>GSHMIARIIGEIGIEGARFIEENIDEQFKALRYLSKGIDSETFVKLVIANSLVSYQLTGKGEQWWWEFAKYFYGRDVKSIYLAYKEFLPNSRFNRRLIPQKLSRIRRVETFLSTLTEERIEEYYGDMSSLWGSIARALGVDKESKTVVF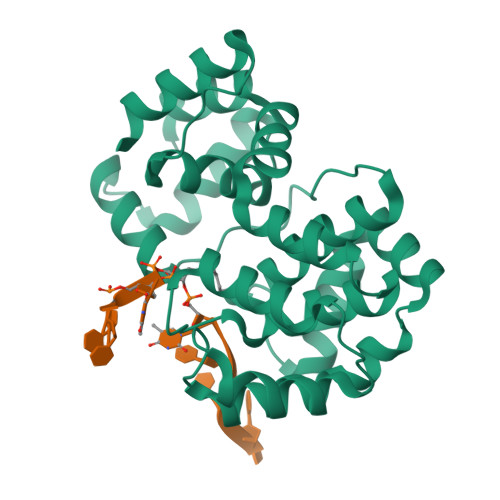SVKMFGYAARIVLSTFNPYPMEIPIPEDSRIVKLTKKLTNEKPRKFWMKIARESGVPPLHIDSILWPLLGGASIDSAPPELRDKLAELIKIIR[4x]>MTTSALPRQAFGEMADTVILLEKATTTPICEGMNRLLASFQALYLQYQKHHFVVEGAEFYPLHQFFQDCYEQVQDHVHALGERLNGLGGVPVAGFQQLAALCCFTPEPEGAFNCRQMLSNDLQAEQAIIGVLRQQATQAESLGDRATAYLYDQILLKTEERAYHIGHFLANDSLKVLKVKLADGREHHH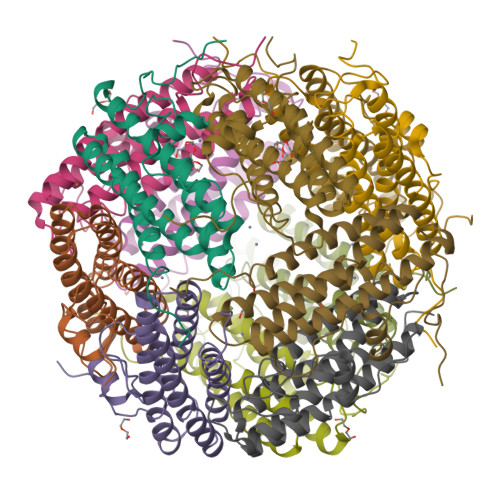HHH[4x]> GNMEASEVMKEKGNAAYKGKQWNKAVNFYTEAIKLNGANATYYCNRAAAFLELCCFQQAEQDCTKAM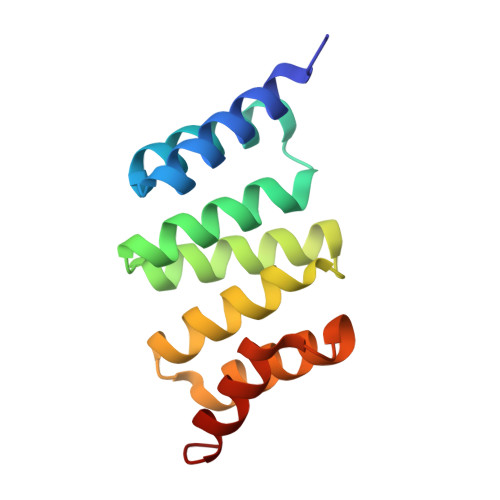LIDKKNVKAYLRRGTAREELVRYKEAAADFRHALVLEPQNKTAKVAEKRLRKHI> GPGSTPVSEKQLAEVVANTITPLMKAQSVPGMAVAVIYQGKPHYYTFGKADIAANKPVTPQTLFELGSISKTFTGVLGGDAIARGEISLDDAVTRYWPQLTGKQWQGIRMLDLATYTAGGLPLQVPDEVTDNASLLRFYQNWQPQWKPGTTRLYANASIGLFGALAVK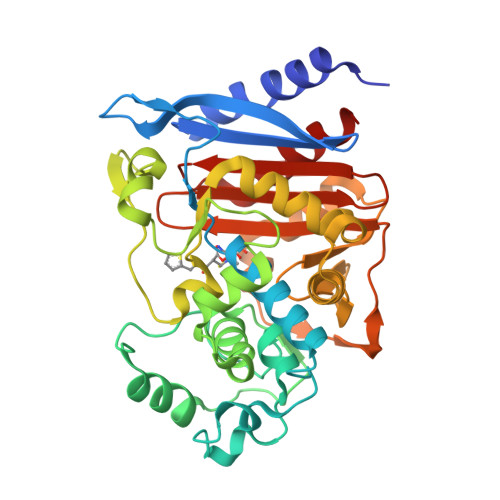PSGMPYEQAMTTRVLKPLKLDHTWINVPKAEEAHYAWGYRDGKAVRVSPGMLDAQAYGVKTNVQDMANWVMANMAPENVADASLKQGIALAQSRYWRIGSMYQGLGWEMLNWPVEANTVVEGSDSKVALAPLPVAEVNPPAPPVKASWVHKTGSTGGFGSYVAFIPEKQIGIVMLANTSYPNPARVEAAYHILEALQ Type IV-A CRISPR-Cas systems diverge from this general mechanism, using a nuclease-independent interference pathway to suppress gene expression for gene regulation and plasmid competition. Here, we present several cryo-EM structures of two evolutionary distant type IV-A1 and type IV-A3 complexes (from Pseudomonas oleovorans and Klebsiella pneumoniae, respectively) bound to cognate DNA targets with and without DinG. The structures reveal multisubunit DNA-surveillance complexes that intimately recognize their DNA-targets to form an R-loop structure. Our results support a model in which DNA-binding is achieved analogously to type I Cascade, while recruitment of DinG differs mechanistically, even in closely related subtypes.

Cryo-EM structure determination of the resulting complexes revealed the effector complexes at average resolutions of ~3.0 Å (type IV-A1) and ~2.9 Å (type IV-A3). Five Cas7 subunits assemble a helical filament along the crRNA spine in type IV-A1, while six subunits form the Cas7-backbone in type IV-A3. The low local resolution of the type IV-A3 effector complex around Cas6 indicates flexibility and prevented model building of Cas6, the predicted crRNA hairpin and some segments of the terminal Cas7.6. However, in type IV-A3, a more pronounced arginine rich loop (RRL; arginines 102, 104, 105 and 110), extending from the Cas5 thumb, inserts into the minor groove of the PAM-adjacent dsDNA. For PAM sequence recognition, Cas8 aligns a loop emanating from its Znf to the minor groove to identify the PAM base pair in position 2, with lysine 79 probing dT2 of the TS. While type IV-A1 stacks a wedge residue onto the PAM base pair in position 0, type IV-A3 Cas8 positions valine 154 and methionine 88 in the minor groove adjacent to the base pair in position 0. Lysine 155 of Cas8 and lysine 119 of Cas5 clamp in place the rotated phosphate that connects the PAM and dG1 of the TS, which together bend the TS for sequence interrogation. Similar to type IV-A1, the structure of type IV-A3 revealed a cryo-EM density corresponding to the NTS (through nucleotide position 8) atop the C-terminal domain of Cas8. Different from type IV-A1, we found α-helices 8 and 9, originating from the thumb domain of Cas7.1, extending from the back of the type IV-A3 effector complex to interlock with the CTD of Cas8. This NTS-interaction mode fully encloses the NTS in a positively charged channel.

>[6x]MRTLNFNGKISTLEPLTVTVKNAVSTSGHRLPRNGGFNAAPYFPGTSIRGTLRHAAHKVIVDRVGLNADGKSPFDLAEHFMLAQGVDINGEAETFAPGEINAGAELRSKNPLISLFGRWGLSGKVGIGNAIPDGDNQWGMFGGGARSIMFQRDESLMEFLETDQVDRLERLLEEQAEASVDISQIKTEQDALKKAMKSADKDTKAELQIKVRELDEKIQARKDQKQESRESIRRPIDPYEAFITGAELSHRMSIKNATDEEAGLFISALIRFAAEPRFGGHANHNCGLVEAHWTVTTWKPGELVPVTLGEIVITPNGVEITGDELFAMVKAFNENQSFDFTARGHHHHHH;> MLNFKPYRVIMSSLTPVVISGIAPSLDGILYEALSQAIPSNEPGVVLARLKEILLFNDELGVFHASSLRFGITPEQGIGATTSMRCDYLSPEKLSTAMFSPRTRRGLFTRVLLTGGPTKRRMTTRPAYSAPYLTFDFVGSSEAVEILLNHAHVGVGYDYFSAANGEFNNVTILPLDIDTSISNEGMALRPVPVNSGLNGIKGVSPLIPPYFVGEKLNIVHPAPVRTQLISSLLRG;> MNHPVESVYSALTSILLPYMGEPVPVQRNCSCCGRAPSEFDGVGFELVNAYRERVVHCRPCQTFFVSAPELMGVENPKKPTTGQKFGMWSGVGAVINVEDNSSVLLAPQGVVNKLPEHFFDHVEVITATSGQHLEYLFNTELKFPLIYIQNFGVKTYELVRSLRVSLSADAIYTCADQLLTRQNEVLYMLDLKKAKELHQEIKNYSKKEMDIFIRTVTLLAYSRITPEAASNEFKKNNLIPLLLLLPTDPHQRLSILHLLKKV(3~{R},4~{R})-4-oxidanyl-3-(phenylmethyl)-4-(phenylmethylsulfanyl)butanoic 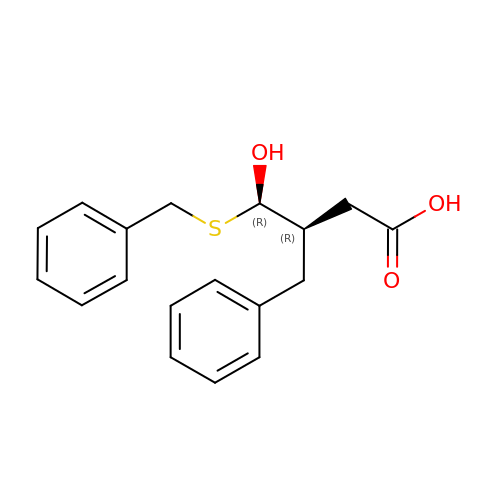acid | C18 H20 O3 S | OBXQOECJZPGJTO-SJLPKXTDSA-N> SQETFSDL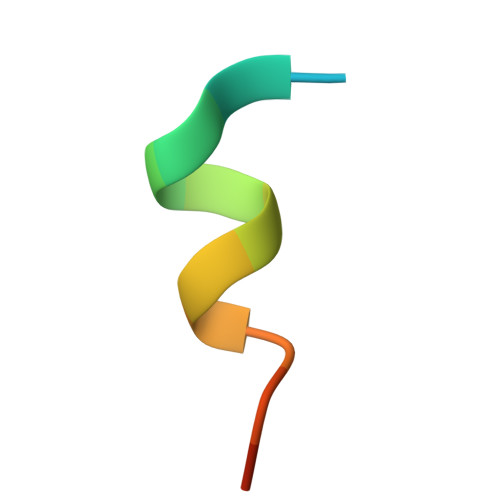WKLLPEN> AVTCPTGQTTANEACCVLFPVIDLLQEELFDGGECGEEAHAALRLAFHDAIGFSKNGGKGGGADGSILAFHQTETTYAANSGIEDIITAQLPIFQKTNLTAGDFVHLAAAIGTGNCPGSPQLA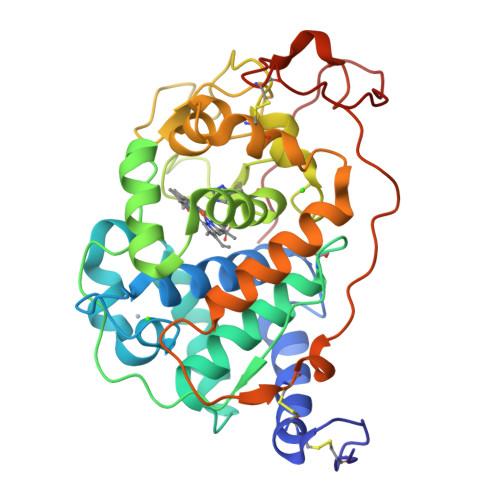YSFGRPPPVAPAPDGTVPEPTDSVTDILARFSEAGFVTAEVIWLLASHSIAAASKIDTSAPRTPFDSTPALFDTQFYLETILNGTLLPGDGGAHTGEVLSPIAGEMRLQSDFAFAQDPRTACLWQEPINDQAFIQGKFFAAMKKLQVLGQTGLTDCSDVIPVPASLPGPITFPAGFSEADVISACTATPLPSLATIAGPKPTIPPVPL Here it is shown which structural adaptations were introduced by directed evolution experiments that changed the catalytic properties of the Escherichia coli (E. coli) (S)-lactaldehyde reductase [EC 1.1.1.77]. This enzyme, referred to as FucO, is also known as an Fe2+, NAD+-dependent group-III alcohol de­hydrogenase and is involved in the catabolism of rare sugars in E. coli.

The mode of binding of NADH in the active site, including the nicotinamide moiety, is well defined by the electron density map, being the same in both structures. Also, crystal structures were obtained of the DA1472 variant in the presence of the bulky substrate analog, compound 7, cocrystallized in the presence of either NAD+ or NADH. The mode of binding of the substrate analog is the same in both structures and well defined by the electron density map. The observed mode of binding of compound 7 is possible because of the N151G and L259V amino acid changes of DA1472. In particular, the side chain of Asn151 of the wild-type active site clashes with the mode of binding of compound 7.

>MMANRMILNETAWFGRGAVGALTDEVKRRGYQKALIVTDKTLVQCGVVAKVTDKMDAAGLAWAIYDGVVPNPTITVVKEGLGVFQNSGADYLIAIGGGSPQDTCKAIGIISNNPEFADVRSLEGLSPTNKPSVPILAIPTTAGTAAEVTIGYVITDEEKRRKFVCVDPHDIPQVAFIDADMMDGMPPALKAATGVDALTHAIEGYITRGAWALTDALHIKAIEIIAGALRGSVAGDKDAGEEMALGQYVAGMGFSNVGVGLVHGMAHPLGAFYNTPHGVANAILLPHVMRYNADFTGEKYRDIARVMGVKVEGMSLEEARNAAVEAVFALNRDVGIPPHLRDVGVRKEDIPALAQAALDDVCTGGNPREATLEDIVELYHTAWTSHHHHH[2x]>[2x]MIFTLRPYQQEAVDATLNHFRRHKTPAVIVLPTG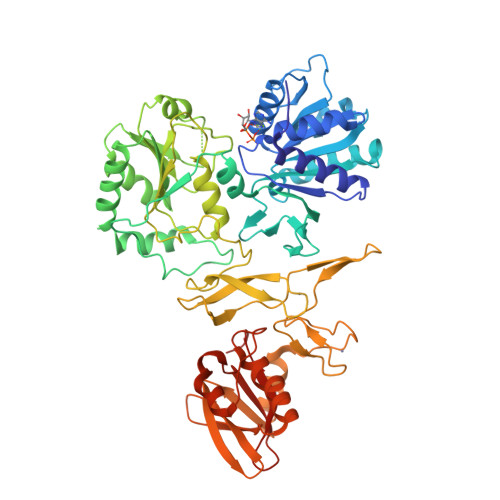AGKSLVIAELARLARGRVLVLAHVKELVAQNHAKYQALGLEADIFAAGLKRKESHGKVVFGSVQSVARNLDAFQGEFSLLIVDECHRIGDDEESQYQQILTHLTKVNPHLRLLGLTATPFRLGKGWIYQFHYHGMVRGDEKALFRDCIYELPLRYMIKHGYLTPPERLDMPVVQYDFSRLQAQSNGLFSEADLNRELKKQQRITPHIISQIMEFAATRKGVMIFAATVEHAKEIVGLLPAEDAALITGDTPGAERDVLIENFKAQRFRYLVNVAVLTTGFDAPHVDLIAILRPTESVSLYQQIVGRGLRLAPGKTDCLILDYAGNPHDLYAPEVGTPKGKSDNVPVQVFCPACGFANTFWGKTTADGTLIEHFGRRCQGWFEDDDGHREQCDFRFRFKNCPQCNAENDIAARRCRECDTVLVDPDDMLKAALRLKDALVLRCSGMSLQHGHDEKGEWLKITYYDEDGADVSERFRLQTPAQRTAFEQLFIRPHTRTPGIPLRWITAADILAQQALLRHPDFVVARMKGQYWQVREKVFDYEGRFRLAHELRG>MGPYRRLWFTLIAVLAVTFALLGFYGGEVYRQAPPIPEEVASADGTRLFGRDDILDGQTAWQSIGGMQLGSIWGHGAYQAPDWTADWLHRELMAWLDLAARDAHGRDYGQLDAPAQAALREQLKAEYRANRADAAGGKLTLSPRRAQAVAQTEAYYDQLFSDAPALHRSRENYAMKENTLPDANRRRQMTHFFFWTAWAAGTEREGTSVTYTNNWPHEPLIGNHPSSENVMWSIISVVVLLAGIGLLIWAWAFLRGKEEDEPPAPARDPLTTFALTPSQRALGKYLFLVVALFGFQVLLGGFTAHYTVEGQKFYGIDLSQWFPYSLVRTWHIQSALFWIATGFLAAGLFLAPLINGGRDPKYQKAGVDILFWALVLVVVGSFAGNYLAIAQIMPPDLNFWLGHQGYEYVDLGRLWQIGKFAGICFWL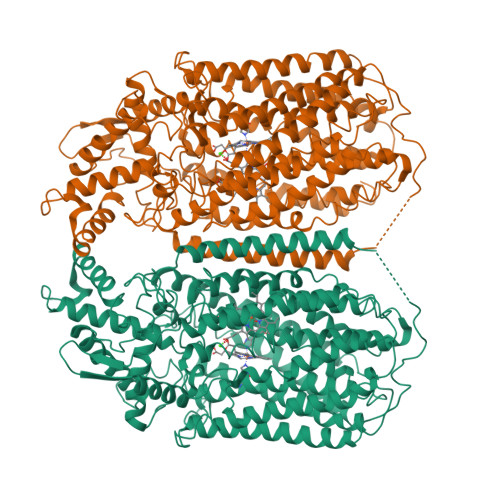VLMLRGIVPALRTPGGDKNLLALLTASVGAIGLFYGAGFFYGERTHLTVMEYWRWWIVHLWVEGFFEVFATTALAFIFSTLGLVSRRMATTASLASASLFMLGGIPGTFHHLYFAGTTTPVMAVGASFSALEVVPLIVLGHEAWENWRLKTRAPWMENLKWPLMCFVAVAFWNMLGAGVFGFMINPPVSLYYIQGLNTTPVHAHAALFGVYGFLALGFTLLVLRYIRPQYALSPGLMKLAFWGLNLGLALMIFTSLLPIGLIQFHASVSEGMWYARSEAFMQQDILKTLRWGRTFGDVVFLLGALAMVVQVILGLLSGK[2x]5'-O-[hydroxy{[hydroxy(phosphonoamino)phosphoryl]oxy}phosphoryl]thymidine 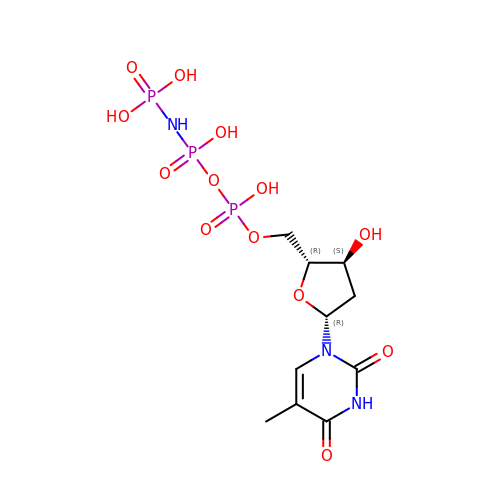| C10 H18 N3 O13 P3 | RTOWUXJWTDSUGC-XLPZGREQSA-N4-hydroxy-3-[(2S,6E,8E)-2-methyldeca-6,8-dienoyl]-5-phenylpyridin-2(1H)-one | C22 H25 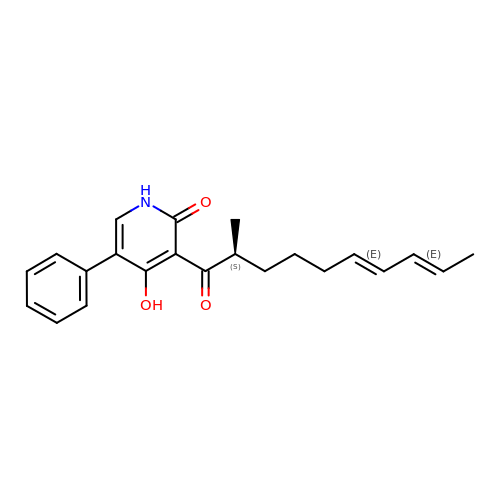N O3 | YJRUCHHILBSMDC-GGXDDXSJSA-N>[2x]MGAMAYPLLLCLLLAQLGLGAVGASRDPQGRPDSPRERTPKGKPHAQQPGRASASDSSAPWSRSTDGTILAQKLAEEVPMDVASYLYTGDSHQLKRANCSGRYELAGLPGKWPALASAHPSLHRALDTLTHATNFLNVMLQSNKSREQNLQDDLDWYQALVWSLLEGEPSISRAAITFSTDSLSAPAPQVFLQATREESRILLQDLSSSAPHLANATLETEWFHGLRRKWRPHLHRRGPNQGPRGLGHSWRRKDGLGGDKSHFKWSPPYLECENGSYKPGWLVTLSSAIYGLQPNLVPEFRGVMKVDINLQKVDIDQCSSDGWFSGTHKCHLNNSECMPIK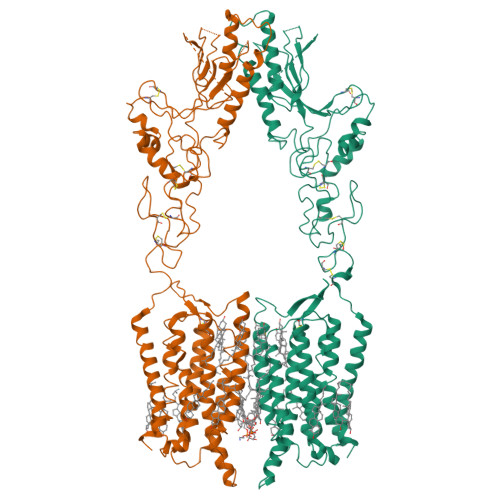GLGFVLGAYECICKAGFYHPGVLPVNNFRRRGPDQHISGSTKDVSEEAYVCLPCREGCPFCADDSPCFVQEDKYLRLAIISFQALCMLLDFVSMLVVYHFRKAKSIRASGLILLETILFGSLLLYFPVVILYFEPSTFRCILLRWARLLGFATVYGTVTLKLHRVLKVFLSRTAQRIPYMTGGRVMRMLAVILLVVFWFLIGWTSSVCQNLEKQISLIGQGKTSDHLIFNMCLIDRWDYMTAVAEFLFLLWGVYLCYAVRTVPSAFHEPRYMAVAVHNELIISAIFHTIRFVLASRLQSDWMLMLYFAHTHLTVTVTIGLLLIPKFSHSSNNPRDDIATEAYEDELDMGRSGSYLNSSINSAWSEHSLDPEDIRDELKKLYAQLEIYKRKKMITNNPHLQKKRCSKKGLGRSIMRRITEIPETVSRQCSKEDKELEVLFQ>[9x]MQRLFLLVAVMLLSGCLTAPPKEAARPTLMPRAQSYKDLTHLPAPTGKIFVSVYNIQDETGQFKPYPASNFSTAVPQSATAMLVTALKDSRWFIPLERQGLQNLLNERKIIRAAQENGTVAINNRIPLQSLTAANIMVEGSIIGYESNVKSGGVGARYFGIGADTQYQLDQIAVNLRVVNVSTGEILSSVNTSKTILSYEVQAGVFRFIDYQRLLEGEVGYTSNEPVMLCLMSAIETGVIFLINDGIDRGLWDLQNKAERQNDILVKYRHMSVPPESWSHPQFEK;>[9x]MRVKHAVVLLMLISPLSWAGTMTFQFRNPNFGGNPNNGAFLLNSAQAQNSYKDPSYNDDFGIETPSALDNFTQAIQSQILGGLLSNINTGKPGRMVTNDYIVDIANRDGQLQLNVTDRKTGQTSTIQVSGLQNNSTDFHHHHHH

Curli are functional amyloids that play critical roles in biofilm formation and adhesion in many Enterobacteriaceae. Two outer membrane proteins, CsgG and CsgF, form the core apparatus for secretion and assembly of the curli structural subunits. In this work, we show that CsgF forms a stable complex with CsgG via a 1:1 stoichiometry by lining the extracellularly faced lumen of the nonameric CsgG channel via its N-terminal 27 residues, creating a secretion channel with 2 constriction regions for curli subunit secretion. The free C-terminal domain of CsgF recruits and binds the secreted nucleator CsgB, creating a growth point for further addition of CsgA subunits.

To improve the resolution of the cryo-EM structure of the CsgG-CsgF complex in order to accurately locate side chains of 9 Asn36 residues of CsgF that consist of the upper constriction region of the CsgG-CsgF channel, the purified CsgG-CsgF complex was proteolytically digested with chymotrypsin to remove flexible regions of the CsgG-CsgF complex that may affect the stability of the complex in the detergent-containing buffers and increase particle heterogeneity on the grid. The resulted protein sample (denoted as the CsgG-CsgF20–59 complex) contained a variant of CsgG that includes residues 47–252 in complex with the most N-terminal 40 residues of the mature CsgF (CsgF20–59), as confirmed by mass spectrometric analysis. In contrast to the oligomerization state exhibited on size exclusion chromatography, the CsgG-CsgF20–59 complexes tended to form filaments with varied lengths on the cryo-EM grids. Intriguingly, there exist 2 types of non-physiological inter-complex interactions: a head-to-head homodimeric interaction and a head-to-tail heterodimeric interaction within the filaments. Using a similar cryo-EM structure determination approach we obtained 2 maps for the nonameric CsgG-CsgF20–53 complex and the nonameric CsgG-CsgF20–59 complex, with an overall resolution of 2.9 Å and 3.2 Å, respectively (S4C, S4D). The structure of the nonameric CsgG-CsgF20–59 complex was obtained from an interacting mode in the filaments through which the most C-terminal 6 residues of each CsgF20–59 fragment interact with the periplasmic regions of each CsgG, stabilizing the conformation of the 6-residue loop of CsgF20–59 in the structure but with relatively weak densities. Structural analysis indicated that formation of the filaments of the CsgG-CsgF20–59 complex on the grids during cryo-EM sample preparation may result from 2 types of inter-complex charge-charge interactions. To test this, we found that increased salt concentrations in the sample buffer significantly decreased the lengths of the filaments formed on the grids.>[2x]MGSSHHHHHHSQDPKPRVLVLTGAGISAESGIRTFRAADGLWEEHRVEDVGTPEGFDRDPELVQAFYNARRRQLQQPEIQPNAAHLALAKLQDALGDRFLLVTQNCDNLHERAGNTNVIHMHGELLKVRCSQSGQALDWTGDVTPEDKCHCCQFPAPLRPHVVWFGEMPLG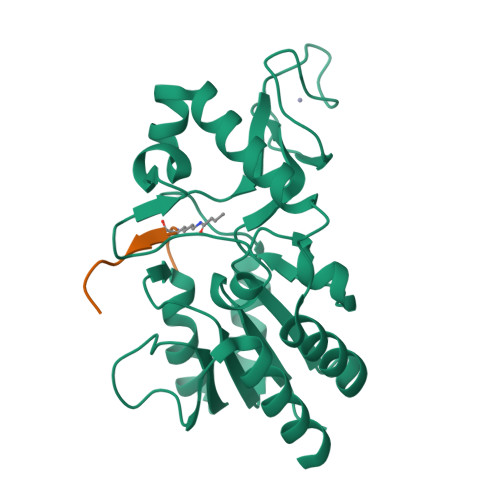MDEIYMALSMADIFIAIGTSGHVYPAAGFVHEAKLHGAHTVELNLEPSQVGNEFAEKYYGPASQVVPEFVEKLLKGLKAGSIA;>[2x]KGGAXRHRKIL> PNFSGNWKIIRSENFEELLKVLGVNVMLRKIWVAAASKPAVEIKQEGDTFYIKVSTTVWTTEINFKVGEEFEEQTVDGRPCKSLVKWESENKMVCEQKLLKGEGPKTSWTKELTNDGELILTMTADDV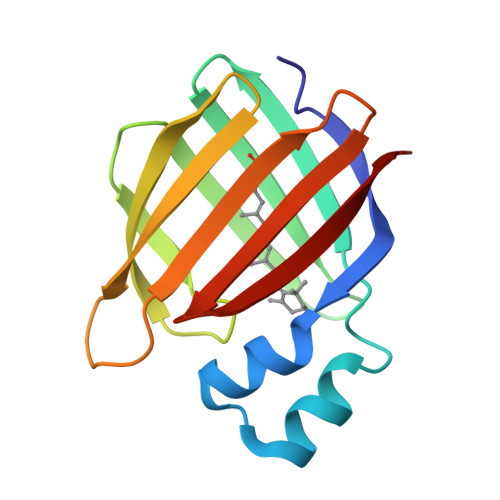VCTLVFVRE O-METHYLCYSTEINE | C4 H9 N O2 S | 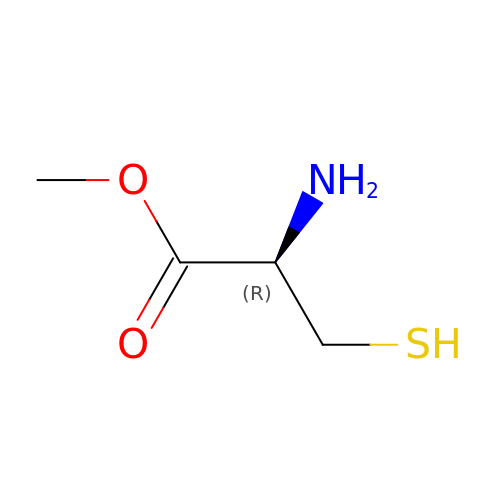MCYHPZGUONZRGO-VKHMYHEASA-N> HHHHHHNKTVLCSNFFTSANRVNCLVPVDGGRKLVYGTDSGIFISERWPKDKSAKPRRVLDASQVTQIDTLEEYQLLLVLANKTLSSYPMEALELAEGQNSVAKRPKKIQGHANFFKAGIGLGRHLVCSVKTSALSSTIKVYEPMDNLAKGKKKSAVSKMFQSGQDTLKPFKEYYIPAESSSIHFLRSTLCVGCARGFEVVSLETTETQSLLDQADTSLDFVARKENVKPIHIERMNGEFLLNYSDFSFFVNRNGWRARPDWKISWEGNPNAFALSYPYILAFEPNFIEIRHIETSELIHIMTGKNIRMLHSSTREILYAYEDEGG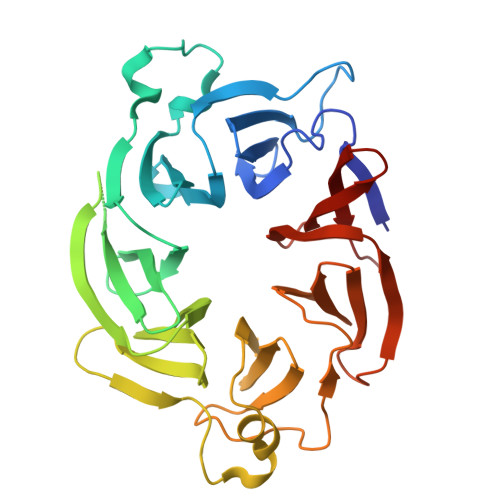EDVVASLDFWNK> LVPRGSHMNTSELRICRINKESGPCTGGEELSLLCDKVQKEDISVVFSTASWEGRADFSQADVHRQIAIVFKTPPYEDLEISEPVTVNVFLQRLTDGVCSEPLPFTYL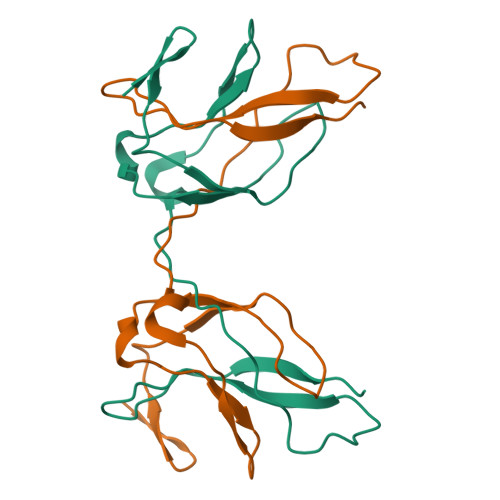PR>[2x]MGSSHHHHHHSQDPNSSSATQGQVITCKAAVAWEPNKPLVIEDVQVAPPQAGEVRVKVLYTALCHTDAYTWSGKDPEGLFPCVLGHEAAGIVESVGEGVTEVQPGDHVIPCYQAECRECKFCKSGKTNLCGKVRAATGVGVMMNDRKSRFSINGKPIYHFMGTSTFSQYTVVHD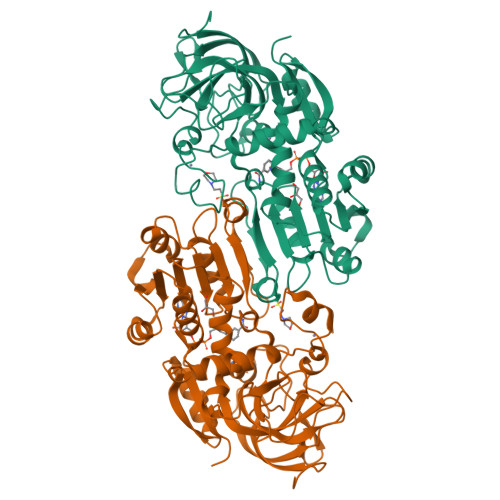VSVAKIDPVAPLEKVCLLGCGVPTGLGAVWNTAKVEPGSIVAVFGLGTVGLAVAEGAKAAGASRIIGIDIDSKKFDRAKNFGVTEFINPKEHEQPIQQVIVDLTDGGVDYSFECIGNVSVMRSALECCHKGWGTSVIVGVAASGQEISTRPFQLVTGRVWKGTAFGGFKSRSQVPSLVDKYLKKEIKVDEYITHNMTLADINKAFDLMHDGDCLRVVLDMFV> METFDQNEVDQILSEFHLQEEDLHVLMCRMQAEMERGLHLETNEEASVKMLPTYVRSTPDGSEVGDFLALDLGGTNFRVMLVKVGEDLEGQWKVETKHKMYSIPVDAMTGTAEMLFDYIAECISDYLDQQNMKHKKLPLGFTFSFPVRHEDIDKGILLNWTKGFKASGAEGNNVVGLLRDAIKRRGDFEMDVVAMVNDTVATMISCYYEDHHCEVGLIVGTGCNACYMEEMSNVELVEGEEGRMCVNTEWGAFGDTGELEDFRLEYDRVVDEASLNPGQQLYEKMIGGKYMGELVRLVLIKMVNENLLFGGESSEKLKTRGAFETQFVSQIEADTSDFKQTLNILRTLGVQATIGDCHAVRLACESVSTRAAIMCSAGLAGILNRMRQSRREELLRITVGVDGSVYKLHPSFKDKFHATVLKLTSGCEITFIQSEEGSGRG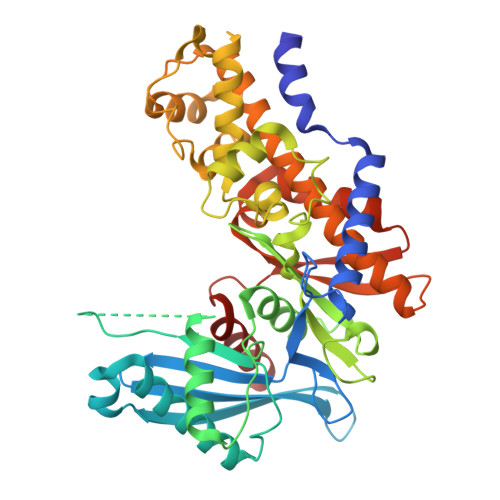AALISAVAYKMAVMIGH>GQDRLDAPPPPAPPLLRWAGPVGVSWGLRAAAPGGPVPRAGRWRRGAPAEDQDCGRLPDFIAKLTNNTHQHVFDDLSGSVSLSWVGDSTGVILVLTTFQVPLVIVSFGQSKLYRSEDYGKNFKDITNLINNTFIRTEFGMAIGPENSGKVILTAEVSGGSRGGRVFRSSDFAKNFVQTDLPFHPLTQMMYSPQNSDYLLALSTENGLWVSKNFGEKWEEIHKAVCLAKWGPNNIIFFTTHVNGSCKADLGALELWRTSDLGKTFKTIGVKIYSFGLGGRFLFASVMADKDTTRRIHVSTDQGDTWSMAQLPSVGQEQFYSILAANEDMVFMHVDEPGDTGFGTIFTSDDRGIVYSKSLDRHLYTTTGGETDFTNVTSLRGVYITSTLSEDNSIQSMITFDQGGRWEHLRKPENSKCDATAKNKNECSLHIHASYSISQKLNVPMAPLSEPNAVGIVIAHGSVGDAISVMVPDVYISDDGGYSWAKMLEGPHYYTILDSGGIIVAIEHSNRPINVIKFSTDEGQCWQSYVFTQEPIYFTGLASEPGARSMNISIWGFTESFITRQWVSYTVDFKDILERNCEEDDYTTWLAHSTDPGDYKDGCILGYKEQFLRLRKSSVCQNGRDYVVAKQPSVCPCSLEDFLCDFGYFRPENASECVEQPELKGHELEFCLYGKEEHLTTNGYRKIPGDKCQGGMNPAREVKDLKKKCTSNFLNPTKQNSKSNAAAHHHHHH[2x]

Sortilin can trigger internalization of ligands from the cell surface via endocytosis and sorts ligands between several intracellular compartments, such as the trans-Golgi network (TGN), endosomes, lysosomes, and the secretory pathway. Sortilin binds and sorts a broad range of ligands, and dysfunction of sortilin has been linked to a wide range of disorders. Previously solved crystal structures of s-sortilin revealed that the Vps10p domain in fact consists of three domains; a ten-bladed β-propeller and two 10CC domains (10CC-a and 10CC-b) that have substantial interactions with the β-propeller. In this study, we detail that sortilin undergoes a conformational change within the three luminal domains and dimerizes while transitioning from neutral to acidic pH.

We determined the structures of the glycosylated luminal segment of mouse sortilin, s-sortilin, from crystals grown at neutral pH (pH 7.5, one crystal form, 2.1 Å maximum resolution) and acidic pH (pH ranging from 5.0 to 6.2, three crystal forms, maximum resolution ranging from 2.3 to 4.0 Å). The structures reveal two distinct conformations, a monomer at neutral pH and a dimer at acidic pH. The eight independent s-sortilin molecules in the three crystal forms grown at acidic pH all form homodimers with an identical interface and highly similar structure. The r.m.s.d. between the s-sortilin chains in the dimers is 0.80 Å for all of the 650 Cα atoms modeled. S-sortilin dimerizes through the top face of the β-propeller, i.e., the large side of the β-propeller disk opposite to the bottom face at which the 10CC domains are located. The predominantly hydrophobic dimer interface is large with a buried surface area of 4882 Å2 and is formed mainly by loops protruding from the blades. β-Propeller blades 1, 4, 6, 7, 8, 9, and 10 are involved in dimer formation. In the s-sortilin dimer the C-termini are in close proximity to each other with 37 Å distance between the two N713 Cα atoms. The s-sortilin dimer structures, crystallized at acidic pH, reveal that dimerization is accompanied by a substantial conformational rearrangement within the ß-propeller and two 10CC domains. Despite three internal disulfide bonds in 10CC-b, the three α-helices that form a small hydrophobic core in the s-sortilin monomer change their conformation into a three-stranded β-sheet in the dimer. In the monomer conformation, the s-sortilin C-terminus is exposed and pointing away from the β-propeller; whereas in the dimer conformation, it is interacting, through conserved hydrophobic interactions, with the rim of the β-propeller at blades 4 and 5.>[4x]MGSSHHHHHHSSGLVPRGSHMASYALNNNSDFNNGWKFTLSDSVCYSFVNYNPSSWKTVNLPHDWSVDLPFESTAEGCTGFLKGGIGWYSKTFDTPDNFVDKKCYIVFDGVYNNSEYWINGRKLGFHPYGYSPFFYDISDYLNPKGQENRISVRIDHSRYADSRWYTGSGIYRETQLIFTDKLHIPVWGTFVTTPVVSSERATVNIEVRVKNDYSGPRAGEVRTSYFDSKNKKVGEKLTSFLIEAGKEMKINQSVEISNPSLWDVDSPSMYLAKSEILVDGNVVDTKETPFGIRSIKFDAKKGFFLNGKNMKIKGVCLHHDASMIGAALVEDVWRRRLQTLKDGGCNA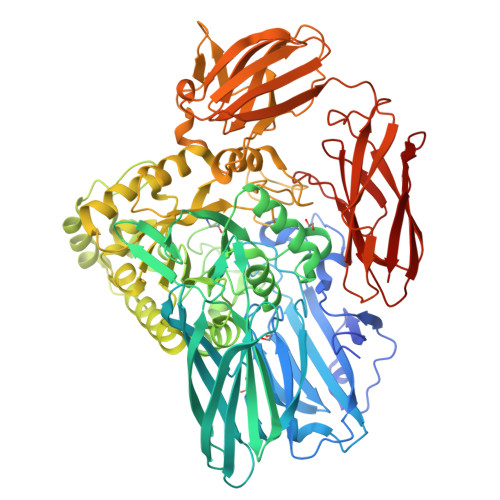IRLSHNPGADAFLELCDEMGFLVQEEFFDEWDYPKDKRLNMDEQSIDYITRGYCEYFQEWAERDLKNVMLRSRNHPCIFQWSIGNEIEWTYKGCKESTGFFSADAGGGYFWNQPPYSTQRIREEWAKQPKQTYDIGRTAKKLAAWTREMDTTRPVTANCILPSISYETGYIDALDVAGFSYRRVMYDYAHKNYPDKPAMGTENLGQWHEWKAVIERDYIPGMFIWTGVDYLGEVGTKGREWPQRAIGCGLLDLAGFEKPSFHMMKSLWTDAPFIAIYSQTANKSSYVEKDGKFTDKDPKKPWTQRLWVWEDVNSHWNYTKGEKVVVEIYSNCDEIELFQNGKSLGKRFLKDFEDHIYKWSVDFKDGNIVAKGKKNGKKTTSAIYTTKETNSIKLSVDKVAVDANNTDVIHVTAQLIDRNGRNISWEEKEITFNIGGNYRLLGVENGDHLNVLNYKSNTVKTYKGRALLVLQATDKAGILNINANSGSISSNDLKVEVK> GTSSMGYLMALFEDIQAVIAEQLNVDAAQVTPEAEFVKDLGADSLDVVELIMALEEKFGIEIPDEQAEKIVNVGDVVKYIED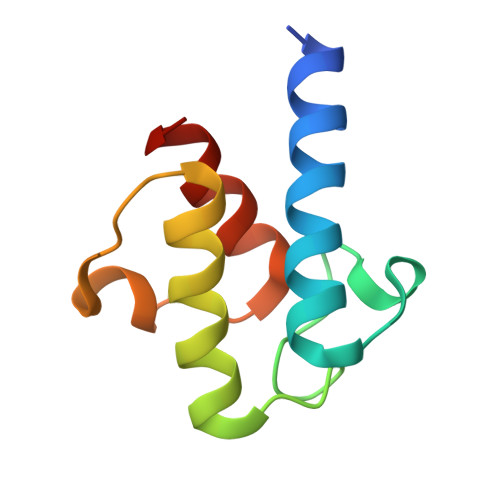NKLA>[2x]MTVQDKAAGSDAEIVTALPVPLAVAGHHQPAPFYLTADMFGGL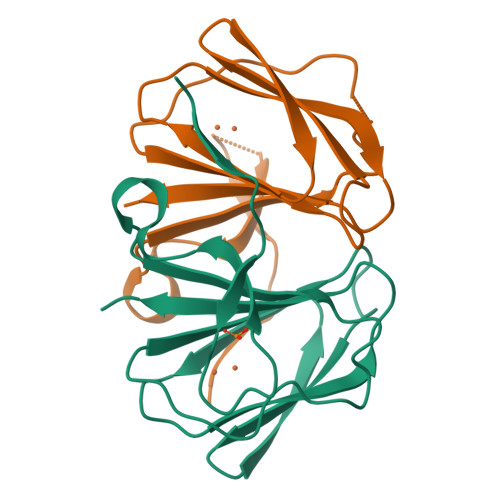PVQLAGGELSKLVGKPVAAPHVHEVDELYFLVSPEPGQARIEVHLDGVRHELVSPAVMRIPAGSEHCFLTLEATVGSYCFGILVGDRL>[2x]MGHMNLTELKNTPVSELITLGENMGLENLARMRKQDIIFAILKQH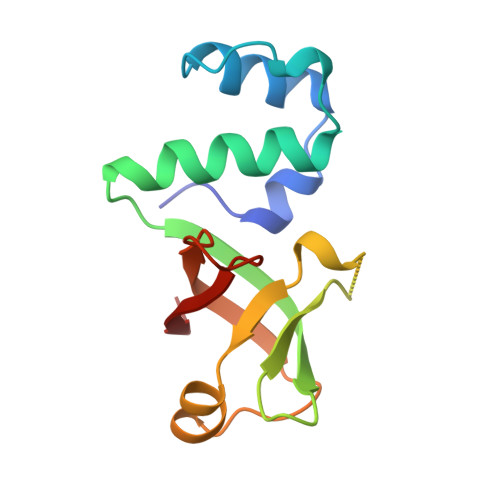AKSGEDIFGDGVLEILQDGFGFLRSADSSYLAGPDDIYVSPSQIRRFNLRTGDTISGKIRPPKEGERYFALLKVNE>[2x]MTEIATTSGARSVGLLSVGAYRPERVVTNDEICQHIDSSDE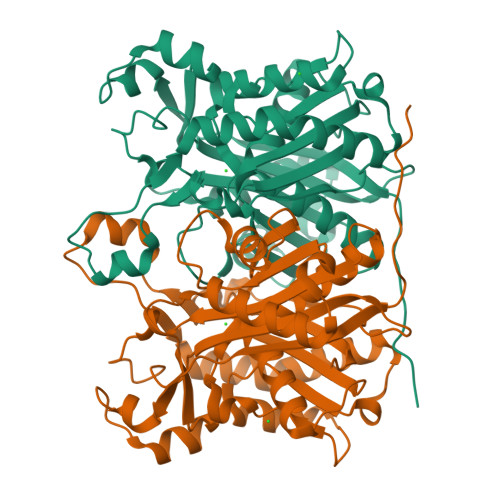WIYTRTGIKTRRFAADDESAASMATEACRRALSNAGLSAADIDGVIVTTNTHFLQTPPAAPMVAASLGAKGILGFDLSAGAAGFGYALGAAADMIRGGGAATMLVVGTEKLSPTIDMYDRGNCFIFADGAAAVVVGETPFQGIGPTVAGSDGEQADAIRQDIDWITFAQNPSGPRPFVRLEGPAVFRWAAFKMGDVGRRAMDAAGVRPDQIDVFVPHQANSRINELLVKNLQLRPDAVVANDIEHTGNTSAASIPLAMAELLTTGAAKPGDLALLIGYGAGLSYAAQVVRMPKG2-azanyl-N-[3-(trifluoromethyloxy)phenyl]ethanamide 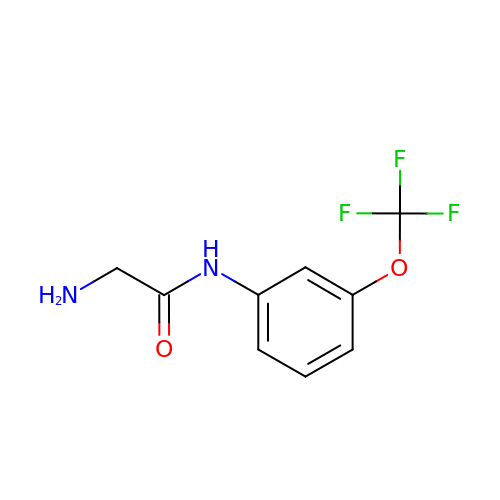| C9 H9 F3 N2 O2 | BZQGZAVHPZXJBL-UHFFFAOYSA-N> VVGGEDAKPGQFPWQVVLNGKVDAFCGGSIVNEKWIVTAAHCVETGVKITVVAGEHNIEETEHTEQKRNVIRIIPHHNYNAAINKYNHDIALLELDEPLVLNSYVTPICIADKEYTNIFLKFGSGYVSGWGRVFHQGQSALVLQYLRVPLVDRATC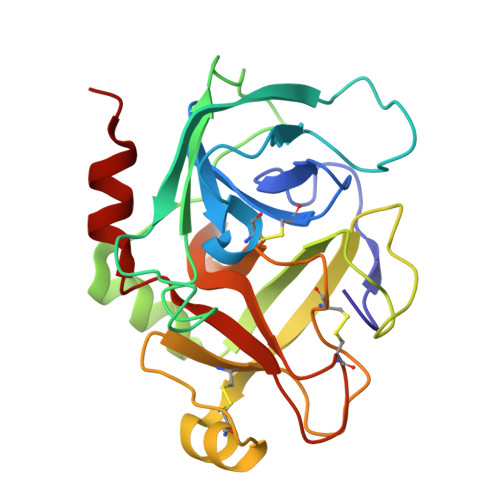LRSTKFTIYNNMFCAGFHEGGRDSCQGDSGGPHVTEVEGTSFLTGIISWGEECAMKGKYGIYTKVSRYVNWIKEKTKLT2-hydroxyethylsulfonic acid | C2 H6 O4 S | 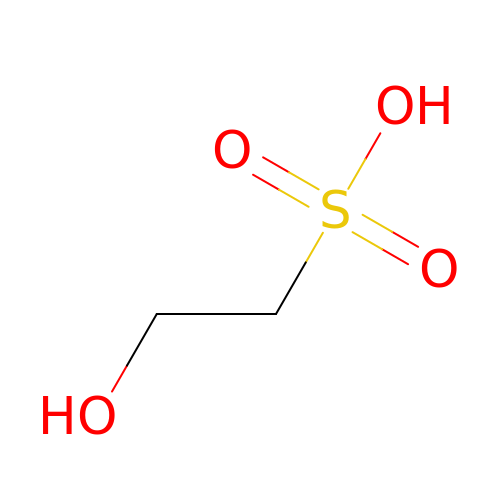SUMDYPCJJOFFON-UHFFFAOYSA-N> MKTQVAIIGAGPSGLLLGQLLHKAGIDNVILERQTPDYVLGRIRAGVLEQGMVDLLREAGVDRRMARDGLVHEGVEIAFAGQRRRIDLKRLSGGKTVTVYGQTEVTRDLMEAREACGATTVYQAAEVRLHDLQGERPYVTFERDGERLRLDCDYIAGCDGFHGISRQSIPAERLKVFERVYPFGWLGLLADTPPVSHELIYANHPRGFALCSQRSATRSRYYVQVPLSEKVEDWSDERFWTELKARLPSEVAEKLVTGPSLEKSIAPLRSFVVEPMQHGRLFLAGDAAHIVPPTGAKGLDLAASDVSTLYRLLLKAYREG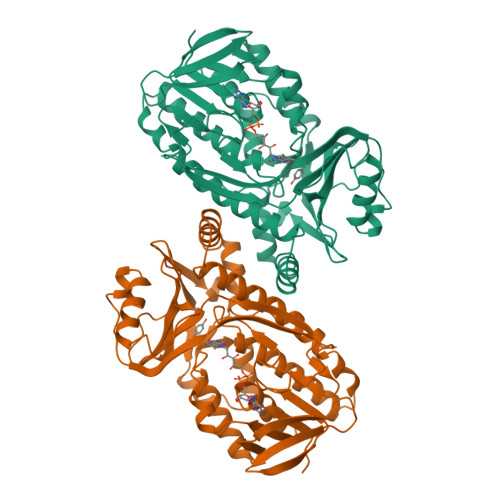RGELLERYSAICLRRIWKAERFSWWMTSVLHRFPDTDAFSQRIQQTELEYYLGSEAGLATIAENYVGLPYEEIE2-[(1R)-2-carboxy-1-(naphthalen-1-ylmethyl)ethyl]-1,3-dioxo-2,3-dihydro-1H-isoindole-5-carboxylic 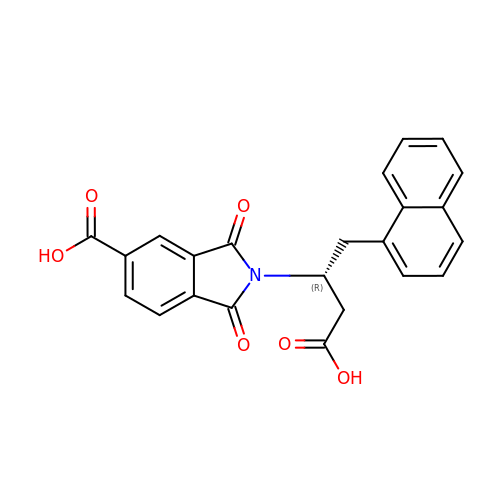acid | C23 H17 N O6 | GPOKTQCDBPECSS-MRXNPFEDSA-N> GPHMAALRPRLVFHTQLAHGSPTGRIEGFTNVKELYGKIAEAFRLPAAEVMFCTLNTHKVDMDKLLGGQIGLEDFIFAHVKGQRKEVEVFKSEEALGLTITDNGAGYAFIKRIKEGSVIDHIQLISVGDMIEAINGQSLLG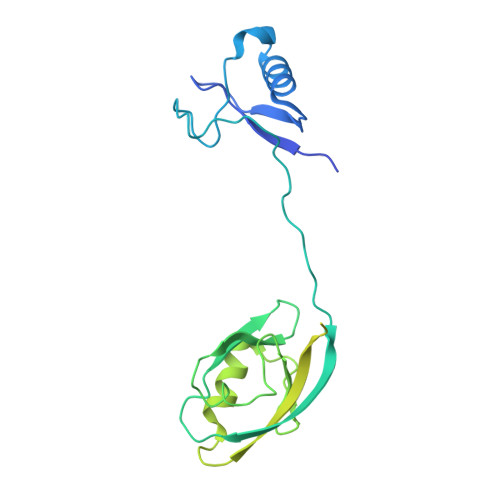CRHYEVARLLKELPRGRTFTLKLTEPRKAFDMISQRSAGGHPGSGPQLGTGRGTLRLRSRGPATVEDLPSAFEEKAIEKVDDLLESYMGIRDTELAATMVELGKDKRNPDELAEALDERLGDFAFPDEFVFDVWGAIGDAKVGRY> GSSRGFPEDSEPISISHGNYTKQYPVFVGHKPGRNTTQRHRLDIQMIMIMNRTLYVAARDHIYTVDIDTSHTEEIYCSKKLTWKSRQADVDTCRMKGKHKDECHNFIKVLLKKNDDTLFVCGTNAFNPSCRNYRVDTLETFGDEFSGMARCPYDAKHANIALFADGKLYSATVTDFLAIDAVIYRSLGDSPTLRTVKHDSKWLKEPYFVQAVDYGDYIYFFFREIAVEYNTMGKVVFPRVAQVCKNDMGGSQRVLEKQWTSFLKARLNCSVPGDSHFYFNILQAVTDVIRINGRDVVLATFSTPYNSIPGSAVCAYDMLDIANVFTGRFKEQKSPDSTWTPVPDERVPKPRPGCCAGSSSLEKYATSNEFPDDTLNFIKTHPLM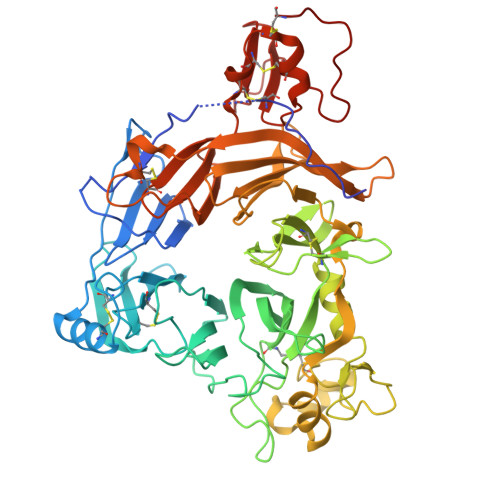DEAVPSIINRPWFLRTMVRYRLTKIAVDNAAGPYQNHTVVFLGSEKGIILKFLARIGSSGFLNGSLFLEEMNVYNPEKCSYDGVEDKRIMGMQLDRASGSLYVAFSTCVIKVPLGRCERHGKCKKTCIASRDPYCGWVRESGSCAHLSPLSRLTFEQDIERGNTDGLGDCHN>[4x]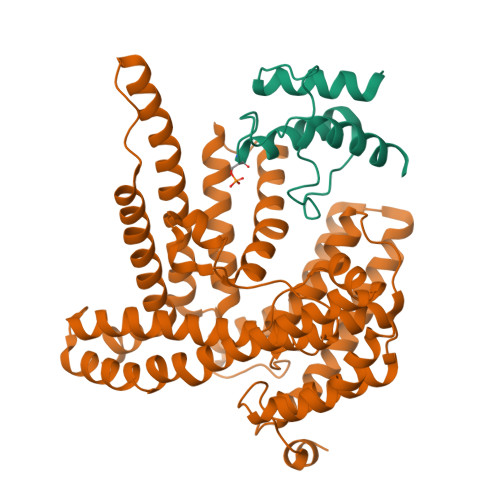GSHMDVKAEVIEIIDELFMEDVSDMMDEDLFDAGVLDSMGTVELIVELESRFDIRVPVSEFGRDDWNTANKIVEGVTELRNA;>[4x]MIDFLKQLPHLEPYGNPFYFIYLGIALLPIFIGLFFKKRFAIYECLVSITFIVLALTGTHASQILALLFYIVWQIIWVYSYKRYRSQRDNKWVFYLHSFLVVLPLILVKVEPTINGTQSLLNFLGISYLTFRAVGMIIEMRDGVLKEFTLGEFLRFMLFMPTFTSGPIDRFKRFNEDYQSIPNRDELLNMLEQAVKYIMLGFLYKFVLAQIFGSMLLPPLKAQALSQGGIFNLPTLGVMYVYGFDLFFDFAGYSMFALAVSNLMGIKSPINFDKPFISRDMKEFWNRWHMSLSFWFRDFVFMRLVIVLMRNKVFKNRNTTSNVAYIINMMVMGFWHGITWYYIAYGIFHGIGLVINDAWLRKKKTINKDRKKAGLKPLPENKWTKALGIFITFNTVMLSFLIFSGFLNDLWFTKKLEHHHHHHHH>SGSSEQELAAIVRDLGCGPYFLGTHDKRFPGFLAGNKLACAIVNTAGRETGGVHWLAFGWNPRSRTCYMFDPFGFSDRRLKQIYSFEYEAMLRRSALALSPDRCLSLEQSTQTVQGPDSAACGLFCCMFLHAFVHWPDRPMDGNPTMNLLTGVPNGMLQSPQVLPTLRRNQEKLYRFLAHHSPYFRSHRAAIEHATAFDKMKQL[2x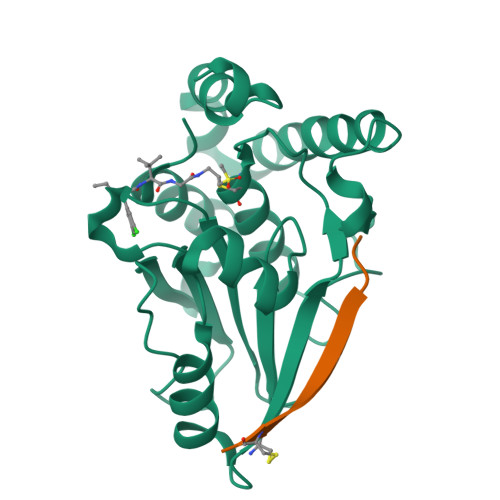];>GVKSLKRRRCY[2x]> SMIDDDGYRPNVGIVICNRQGQVMWARRFGQHSWQFPQGGINPGESAEQAMYRELFEEVGLSRKDVRILASTRNWLRYKLPKRLVRWDTKPVCIGQKQKWFLLQLVSGDAEINMQTSSTPEFDGWRWVSYWYPVRQVVSFKRDVYRRVMAAFASVVMSLQE

Finding a correct substrate is especially difficult for the Escherichia coli Nudix hydrolase RppH, which triggers 5′-end-dependent RNA degradation by removing orthophosphate from the 5′-diphosphorylated transcripts. In Escherichia coli and probably many other bacteria, RppH converts diphosphorylated 5′ ends of transcripts into monophosphorylated ends that accelerate subsequent cleavage by the 5′-monophosphate-stimulated endonuclease RNase E. Escherichia coli RppH can also remove pyrophosphate from triphosphorylated RNA with lower efficiency. Here we show that RppH binds and slowly hydrolyzes NTPs, NDPs and (p)ppGpp, which each resemble the 5′-end of RNA. A series of X-ray crystal structures of RppH-nucleotide complexes, trapped in conformations either compatible or incompatible with hydrolysis, explain the low reaction rates of mononucleotides and suggest two distinct mechanisms for their hydrolysis.

To understand how nucleotides inhibit the reaction of RppH with the RNA substrates, we determined 1.6–1.9 Å crystal structures of RppH bound to triphosphorylated nucleosides and/or their non-hydrolysable analogs, ppcpNs, which contain a methylene moiety instead of a bridging oxygen atom between α- and β-phosphates. Neither structure contains Mg2+ cations since their addition to the crystallization solution resulted in the loss of electron density map for nucleotides, even for non-hydrolysable substrate analogs and at pH values unfavorable for catalysis. In the absence of Mg2+, the map for nucleotides was of high quality although the occupancy of nucleotides was refined to lower than 100% in some cases. In all of the structures, the position of the nucleobases is nearly invariant, while the conformations of the sugar–phosphate moieties have small differences. All of the nucleobases bind in the protein cleft where we previously observed specific binding of guanosine at the second position of an RNA ligand. In this cleft, the nucleobase is sandwiched between the guanidinium group of R27 and a hydrophobic pedestal formed by V137 and F139. Pyrimidines are locked in place by a hydrogen bond with S32, while purines are likely held by stronger cation–π interactions with R27. The sugar–phosphate moiety is oriented toward the catalytic site and forms several hydrogen bonds involving R27, Y77, Q95 and K140 in all of the structures. Thus, the NTP-bound structures demonstrate that NTPs interact with RppH in the same site where the second nucleotide of RNA binds RppH. In this position, NTPs can compete with RNA for RppH binding and inhibit the reaction of RNA substrates.> MSKMSDVKCTSVVLLSVLQQLRVESSSKLWAQCVQLHNDILLAKDTTEA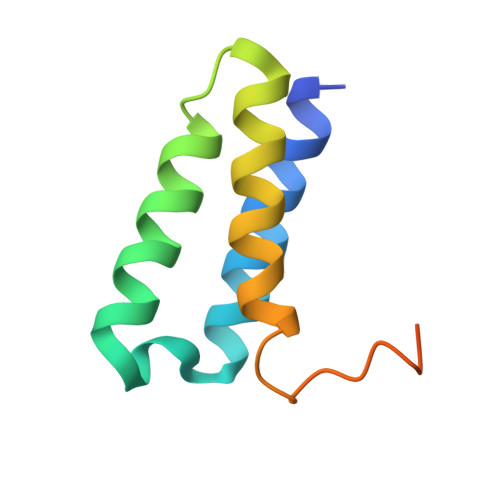FEKMVSLLSVLLSMQGAVDINKLCEEMLDNRATLQ>[3x]MSQFFIRRPVFAWVIAIFII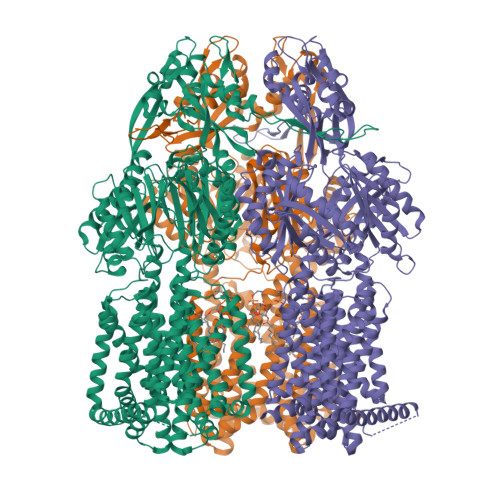IFGLLSIPKLPIARFPSVAPPQVNISATYPGATAKTINDSVVTLIERELSGVKNLLYYSATTDTSGTAEITATFKPGTDVEMAQVDVQNKIKAVEARLPQVVRQQGLQVEASSSGFLMLVGINSPNNQYSEVDLSDYLVRNVVEELKRVEGVGKVQSFGAEKAMRIWVDPNKLVSYGLSISDVNNAIRENNVEIAPGRLGDLPAEKGQLITIPLSAQGQLSSLEQFKNISLKSKTNGSVIKLSDVANVEIGSQAYNFAILENGKPATAAAIQLSPGANAVKTAEGVRAKIEELKLNLPEGMEFSIPYDTAPFVKISIEKVIHTLLEAMVLVFIVMYLFLHNVRYTLIPAIVAPIALLGTFTVMLLAGFSINVLTMFGMVLAIGIIVDDAIVVVENVERIMATEGLSPKDATSKAMKEITSPIIGITLVLAAVFLPMAFASGSVGVIYKQFTLTMSVSILFSALLALILTPALCATILKPIDGHHQKKGFFAWFDRSFDKVTKKYELMLLKIIKHTVPMMVIFLVITGITFAGMKYWPTAFMPEEDQGWFMTSFQLPSDATAERTRNVVNQFENNLKDNPDVKSNTAILGWGFSGAGQNVAVAFTTLKDFKERTSSASKMTSDVNSSMANSTEGETMAVLPPAIDELGTFSGFSLRLQDRANLGMPALLAAQDELMAMAAKNKKFYMVWNEGLPQGDNISLKIDREKLSALGVKFSDVSDIISTSMGSMYINDFPNQGRMQQVIVQVEAKSRMQLKDILNLKVMGSSGQLVSLSEVVTPQWNKAPQQYNRYNGRPSLSIAGIPNFDTSSGEAMREMEQLIAKLPKGIGYEWTGISLQEKQSESQMAFLLGLSMLVVFLVLAALYESWAIPLSVMLVVPLGIFGAIIAIMSRGLMNDVFFKIGLITIIGLSAKNAILIVEFAKMLKEEGMSLIEATVAAAKLRLRPILMTSLAFTCGVIPLVIATGASSETQHALGTGVFGGMISATILAIFFVPVFFIFILGAVEKLFSSKKKISS> PSMMPQWSYMHISGQDASEYLSPGLVQFARATETYFSLNNKFRNPTVAPTHDVTTDRSQRLTLRFIPVDREDTAYSYKARFTLAVGDNRVLDMASTYFDIRGVLDRGPTFKPYSGTAYNALAPKGAPNPCEWDEAATALEINLEEEDDDNEDEVDEQAEQQKTHVFGQAPYSGINITKEGIQIGVEGQTPKYADKTFQPEPQIGESQWYETEINHAAGRVLKKTTPMKPCYGSYAKPTNENGGQGILVKQQNGKLESQVEMQFFSTTEATAGNGDNLTPKVVLYSEDVDIETPDTHISY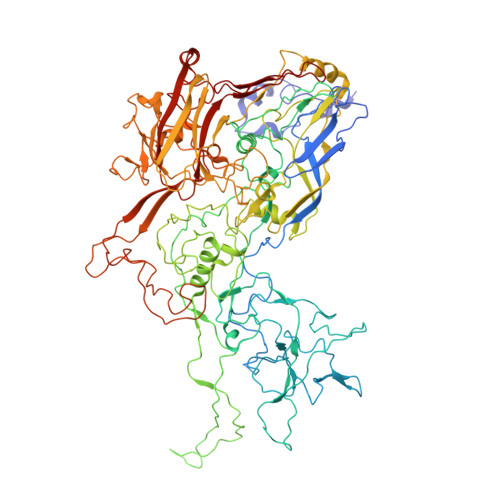MPTIKEGNSRELMGQQSMPNRPNYIAFRDNFIGLMYYNSTGNMGVLAGQASQLNAVVDLQDRNTELSYQLLLDSIGDRTRYFSMWNQAVDSYDPDVRIIENHGTEDELPNYCFPLGGVINTETLTKVKPKTGQENGWEKDATEFSDKNEIRVGNNFAMEINLNANLWRNFLYSNIALYLPDKLKYSPSNVKISDNPNTYDYMNKRVVAPGLVDCYINLGARWSLDYMDNVNPFNHHRNAGLRYRSMLLGNGRYVPFHIQVPQKFFAIKNLLLLPGSYTYEWNFRKDVNMVLQSSLGNDLRVDGASIKFDSICLYATFFPMAHNTASTLEAMLRNDTNDQSFNDYLSAANMLYPIPANATNVPISIPSRNWAAFRGWAFTRLKTKETPSLGSGYDPYYTYSGSIPYLDGTFYLNHTFKKVAITFDSSVSWPGNDRLLTPNEFEIKRSVDGEGYNVAQCNMTKDWFLVQMLANYNIGYQGFYIPESYKDRMYSFFRNFQPMSRQVVDDTKYKDYQQVGILHQHNNSGFVGYLAPTMREGQAYPANFPYPLIGKTAVDSITQKKFLCDRTLWRIPFSSNFMSMGALTDLGQNLLYANSAHALDMTFEVDPMDEPTLLYVLFEVFDVVRVHRPHRGVIETVYLRTPFSAGNATT>[2x]DRIKANPVSEKNIDEKFIYNTADFSIELFKNSIDDKENSLISPLSAMLALAMTANGADNETLAQMEKALGKDISIEDLNKYLYTYMKKLPNEEKSKLTIANSIWFKENDFMPSKDFLQIIADYYKADIFKAAFDSSTVSDINNWVKSKTNGMIDKILNKIDPEDVMYLINAVAFDAEWETVYEKASVHEDIFTDVY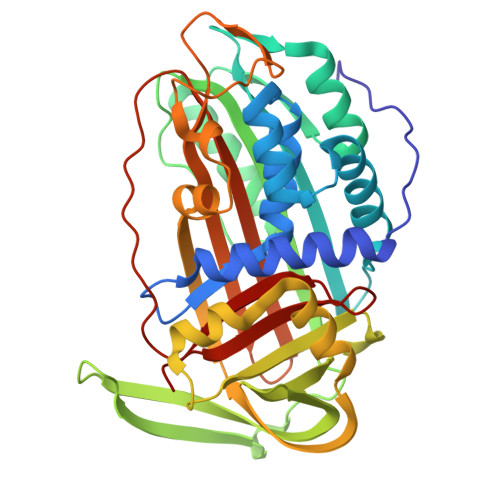GNRQKVEFMNSEENLYIEEENAIGFVKPYAKNHYSFVAILPDENISVNEYIKTLTGQKFIDLIKNAKITLVRASLPKFKYEYTIKMNETLESLGMTDAFLPDKADFSKLGKSDIGNLYISEVLHKTFISVDELGTKAGAVTSVDITAAGIPVNFKTVKLNRPFIFAIIDNSTNLPIFIGTVLSLK>[7x]XGEIAQALKEIAKALKEIAWALKEIA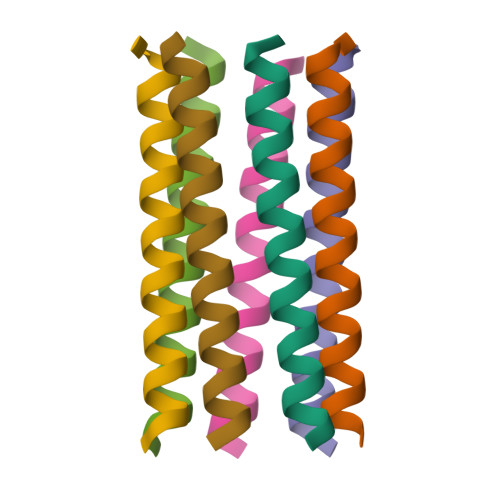QAYKGX> MKKIANYLLIEKTD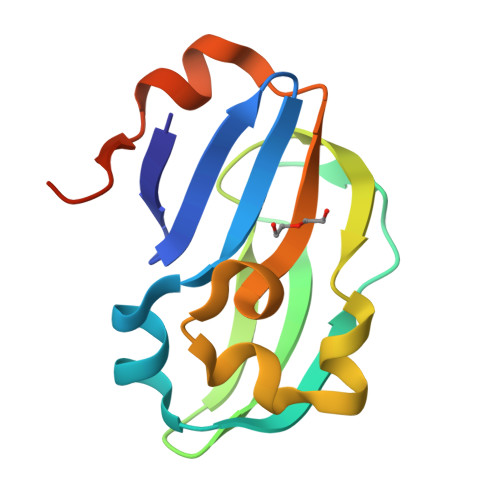DRYTISMTPELQDDIGTIGYAEFTDNDHLAVDDIILNLEASKTVMSVLSPLAGAVVERNEAATLTPTLLNSEKAEENWIVVLTDVDQAAFDALEDAGSGHHHHHHH>[3x]MTTTRTERNFAGIGDVRIVYDVWTPDTAPQAVVV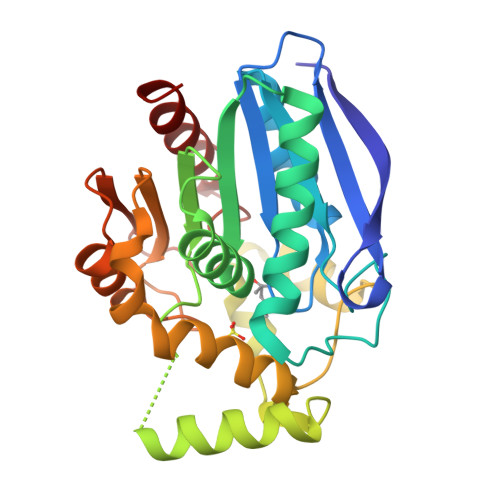LAHGLGEHARRYDHVAQRLGAAGLVTYALDHRGHGRSGGKRVLVRDISEYTADFDTLVGIATREYPGCKRIVLGHSMGGGIVFAYGVERPDNYDLMVLSAPAVAAQDLVSPVVAVAAKLLGVVVPGLPVQELDFTAISRDPEVVQAYNTDPLVHHGRVPAGIGRALLQVGETMPRRAPALTAPLLVLHGTDDRLIPIEGSRRLVECVGSADVQLKEYPGLYHEVFNEPERNQVLDDVVAWLTERL>MGSHHHHHHENLYFQGHMNSFYSQEELKKIGFLSVGKNVLISKKASIYNPGVISIGNNVRIDDFCILSG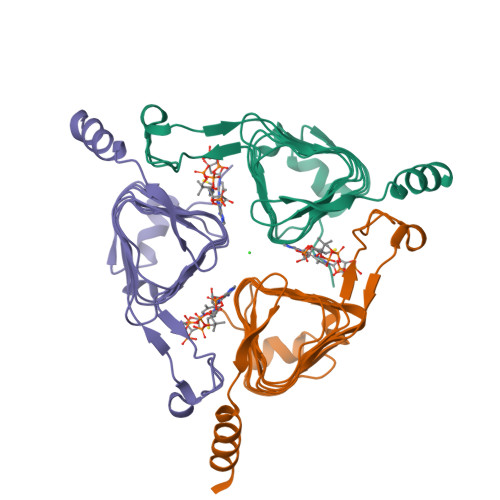KVTIGSYSHIAAYTALYGGEVGIEMYDFANISSRTIVYAAIADFSGNALMGPTIPNQYKNVKTGKVILKKHVIIGAHSIIFPNVVIGEGVAVGAMSMVKESLDDWYIYVGVPVRKIKARKRKIVELENEFLKSMNS[3x]> FACKTANGTAIPIGGGSANVYVNLAPVVNVGQNLVVDLSTQIFCHNDYPETITDYVTLQRGSAYGGVLSNFSGTVKYSGSSYPFPTTSETPRVVYNSRTDKPWPVALYLTPVSSAGGVAIKAGSLIAVLILRQTNNYNSDDFQFVWNIYANNDVVVPTGGCDVSARDVTVTLPDYRGSVPIPLTVYCAKSQNLGYYLSGTHADAG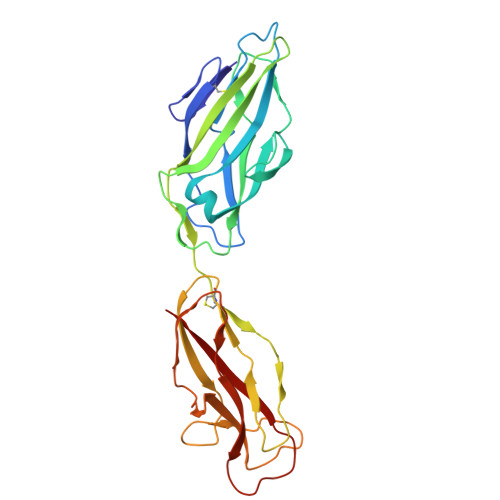NSIFTNTASFSPAQGVGVQLTRNGTIIPANNTVSLGAVGTSAVSLGLTANYARTGGQVTAGNVQSIIGVTFVYQ>MADIYPLGKTHTEELNEIIVESAKEIAEPDTTMIQKLIDEHNPEPLLKGVRYYMCENDIEKKRRTYYDAAGQQLVDDTKTNNRTSHAWHKLFVDQKTQYLVGEPVTFTSDNKTLLEYVNELADDDFDDILNETVKNMSNKGIEYWHPFVDEEGEFDYVIFPAEEMIVVYKDNTRRDILFALRYYSYKGIMGEETQKAELYTDTHVYYYEKIDGVYQMDYSYGENNPRPHMTKGGQAIGWGRVPIIPFKNNEEMVSDLKFYKDLIDNYDSITSSTMDSFSDFQQIVYVLKNYDGENPKEFTANLRYHSVIKVSGDGGVDTLRAEIPVDSAAKELERIQDELYKSAQAVDNSPETIGGGATGPALEKLYALLDLKANMAERKIRAGLRLFFWFFAEYLRNTGKGDFNPDKELTMTFTRTRIQNDSEIVQSLVQGVTGGIMSKETAVARNPFVQDPEEE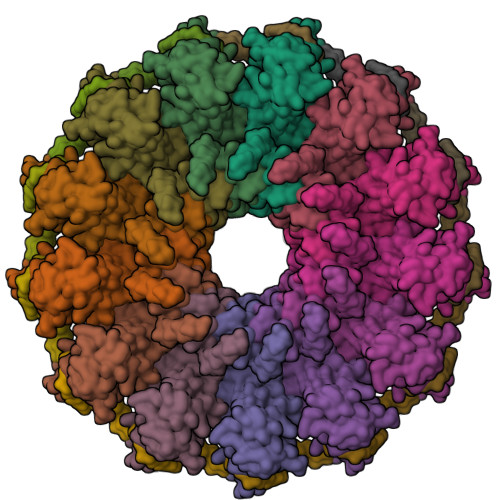LARIEEEMNQYAEMQGNLLDDEGGDDDLEEDDPNAGAAESGGAGQVS[13x]>MKKFPEGFLWGVATASYQIEGSPLADGAGMSIWHTFSHTPGNVKNGDTGDVACDHYNRWKEDIEIIEKIGAKAYRFSISWPRILPEGTGKVNQKGLDFYNRIIDTLLEKNITPFITIYHWDLPFSLQLKGGWANRDIADWFAEYSRVLFENFGDRVKHWITLNELWVVAIVGHLYGVHAPGMKDIYVAFHTVHNLLRAHAKSVKVFRETVKDGKIGIVFNNGYFEPASEREEDIRAARFMHQFNNYPLFLNPIYRGEYPDLVLEFAREYLPRNYEDDMEEIKQEIDFVGLNYYSGHMVKYDPNSP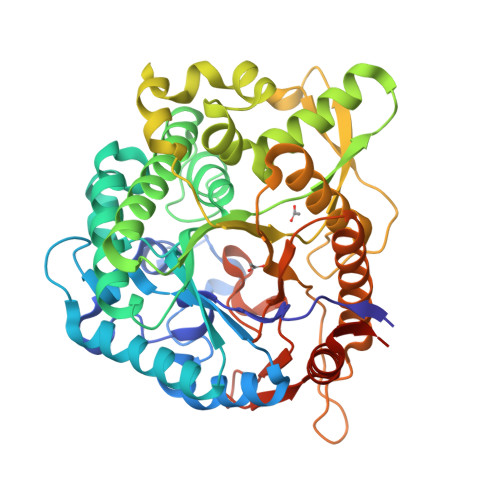ARVSFVERNLPKTAMGWEIVPEGIYWILKGVKEEYNPQEVYITGNGAAFDDVVSEGGKVHDQNRIDYLRAHIEQVWRAIQDGVPLKGYFVWSLLDNFEWAEGYSKRFGIVYVDYNTQKRIIKDSGYWYSNVIKNNGLTDLEHHHHHH[2x]>[2x]GAMGKSEGVTIEFKIVGLNKKLKVFTTCPHTLFGASFCAVAIEHPIVQDLMSKEIQDLISSIKIQGKNNEKVGIYTGLNVKHPFLDKELPLYVANFVLMEYREGAIFGCPAHDQRDFEFAQEYDLPIIPVISSARLGIEEYTNNSIMFNSEFLNGLTVSEARKVIVEKLEEKGIGKKTI

Here, we report the discovery of potent boron-based compounds that inhibit an unprecedented target of Wolbachia, leucyl-tRNA synthetase (LeuRS), and demonstrate that inhibition of this microbiota target is an efficient approach to arrest the growth of its host. The editing site of LeuRS plays a key role to maintain fidelity in protein translation by hydrolyzing tRNALeu mischarged to noncognate amino acids such as norvaline. Altogether, these experiments show that benzoxaborole inhibitors of Wolbachia LeuRS are prodrugs that, in an enzyme-independent manner, form adducts with adenosine substrates. The adducts then bind with potent nanomolar affinity into the Wolbachia LeuRS editing site and efficiently compete with the physiological substrate norvaline.

In the absence of AMP, Cmpd6 and Cmpd9 did not bind to Wolbachia LeuRS; however, in the presence of AMP, the compounds were potent LeuRS inhibitors, with dissociation constants of 44 and 6 nM, respectively. Cmpd9 has stronger affinity than Cmpd6, which arises from a more favorable binding entropy, likely due to a more optimal conformation by the alkyl-phenyl group of Cmpd9 to bind into the Wolbachia LeuRS drug pocket. The potent nanomolar affinities of the two compounds are explained by a combination of multiple polar and hydrophobic interactions established by the inhibition adducts in the editing site. Both compounds make equivalent interactions with Wolbachia LeuRS, except for minor differences in the 2-amido-thiazole and amino-methyl phenyl groups of Cmpd6 and Cmpd9, respectively. Specifically, the amino-methyl phenyl of Cmpd9 packs between residues F311, L313, and Y316, and makes several hydrophobic contacts, and at the same time, the phenyl group makes two favorable aromatic π-π interactions, one parallel-displaced with the adenosine ring and one T-shape stacking with Y316. This conformation is further stabilized by hydrogen bonds of the adenosine-phosphate to residues Y316 and S221. Other key interactions, shared by the two compounds, are a hydrogen bond by the oxaborole oxygen-1 to T241; and the three hydrogen bonds established by the 3-aminomethyl to F322, D328, and D331. In the adduct formed with AMP, the phenyl and amido-thiazole groups stack against the adenosine base and enable multiple interactions within the Wolbachia LeuRS drug pocket. Conversely, the B factors of the adduct AMP-Cmpd9 are invariably low for all atoms, including the phenyl group.> KPEFDPILLRPVDD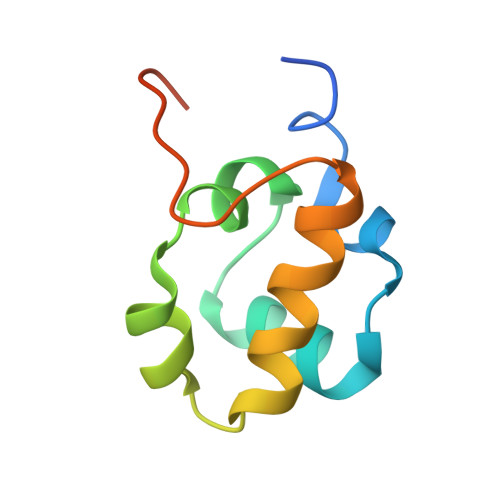LELTVRSANCLKAEAIHYIGDLVQRTEVELLKTPNLGKKSLTEIKDVLASRGLSLGMRLENWPPASIADE> MHMKNIKKNQVMNLGPNSKLLKEYKSQLIELNIEQFEAGIGLILGDAYIRSRDEGKTYCMQFEWKNKAYMDH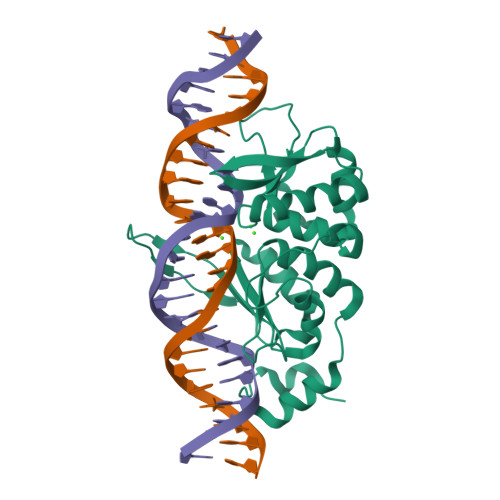VCLLYDQWVLSPPHKRERVNHLGNLVITWTAQTFKHQAFNKLANLFIVNNKKTIPNNLVENYLTPMSLAYWFMDDGGKWDYNKNSTNKSIVLNTQSFTFEEVEYLVKGLRNKFQLNCYVKINKNKPIIYIDSMSYLIFYNLIKPYLIPQMMYKLPNTISSETFLK>MKILVTGAAGFIGSHLCQALLKNSAYHVVGIDHFIGPTPATLKTGNIQSLELNSRFQFIREDILNTDLSKLLQDIDVVYHLAAIPGVRTSWGKDFQPYVTNNIMVTQQLLEACKHIKLDKFIHISTSSVYGEKSGAVSEDLLPIPLSPYGVTKLSGEHLCHVYHKNFHIPIVILRYFTVYGPRQRPDMAFHRLIKQMLEDKPLTIFGDGTQTRDFTYIDDCIRGTVAALETKKNIIGEVINIGGKEQASILDIISMLEKISGKS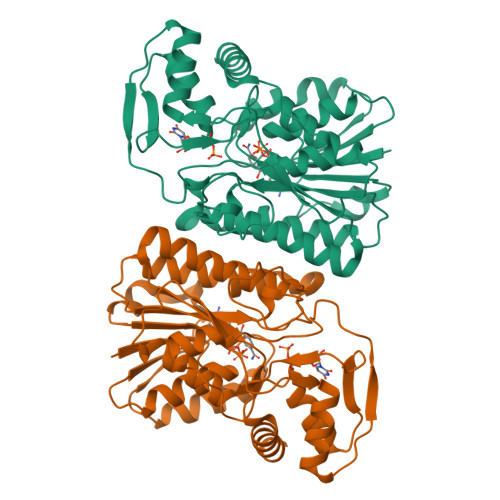ATKNFLKSVPGEPKQTWADISKASTLLQYSPTVSLSDGLEAEYDYIKQLYKGDAAWSHPQFEK[2x]>[2x]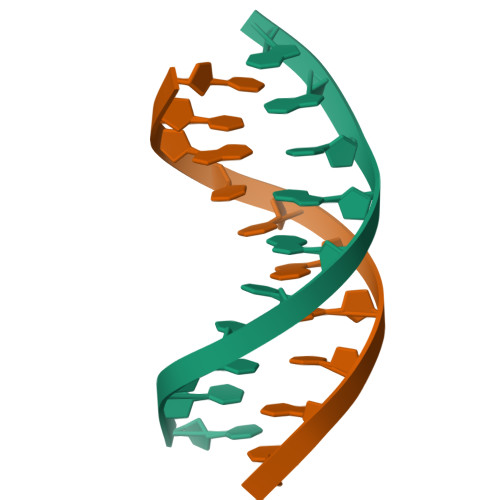CCATTAATGG>[2x]AEYSKV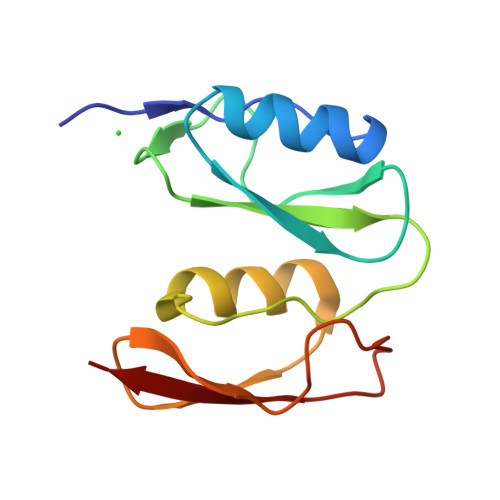PDVEGQDKQKAIDNVSAKSLEPVTIGSGTQIKAQSIKAGNKVLPHSKVLLLTDGDLTMPDMSGWTKEDVIAFENLTNIKVNLKGSGFVSHQSISKGQKLTEKDKIDVEFSS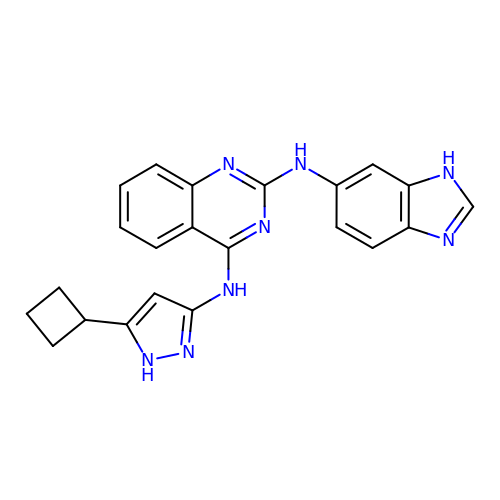N~2~-(1H-benzimidazol-6-yl)-N~4~-(5-cyclobutyl-1H-pyrazol-3-yl)quinazoline-2,4-diamine | C22 H20 N8 | DLCOOKRUECVLCI-UHFFFAOYSA-N>[6x]MKILVIQGPNLNMLGHRDPRLY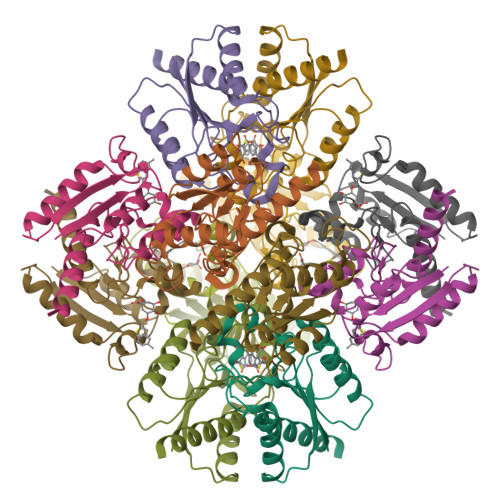GMVTLDQIHEIMQTFVKQGNLDVELEFFQTNFEGEIIDKIQESVGSDYEGIIINPGAFSHTSIAIADAIMLAGKPVIEVHLTNIQAREEFRKNSYTGAACGGVIMGFGPLGYNMALMAMVNILAEMKAFQEAQKNNPNNPINNQK>MGEEVNFDWHLLLNGYYYSPVDLEVEDIFEIVNQPMDGNCLYHSLACGMIEEQQPDSYKLIKEQVREAAGLFWDTTEETKTTGEDLNGYLARIMKPNEWGSSLEVNFFSQKAKVTVYIWHEDASKHCDYVVRYGEDPMLESINIMHRRNHYDYLKPRGNQRTAVVKSGSHHHHHH[4x]

One specific mechanism used by nairoviruses is the production of a deubiquitinating enzyme, termed the vOTU, that disrupts the innate immune response. Interestingly, the nairoviral L segment also encodes a viral homologue of the ovarian tumor protease (OTU) at the N-terminus. Instead, the vOTU’s primary function appears to be the reversal of post-translational modifications by ubiquitin (Ub) and the Ub-like protein interferon stimulated gene product 15 (ISG15). Each vOTU possesses a seven-stranded beta sheet as the core feature, with five major alpha helices framing the rest of the structure.

The vOTUs from DGKV, QYBV, and TAGV readily crystallized and were solved to 1.62 Å, 1.65 Å, and 2.05 Å, respectively. TAGV vOTU, on the other hand, prefers K63 and K11 to a greater extent, while not possessing as much activity towards K48. In TAGV vOTU, Trp73 fits between Leu86 and Thr79. Similarly, for TAGV vOTU Thr76 and Glu78 form electrostatic interactions with Gln110 and Tyr133, respectively. In TAGV vOTU, this pocket is largely hydrophobic possessing two tyrosines as well as a valine. Looking at X-ray crystal structures of the CCHFV and DUGV vOTUs bound to Ub reveals that Leu8 in particular has to be spatially accommodated in a pocket deep within the interaction interface. To confirm that this interaction with Leu8 is likewise involved in Ub binding with these other vOTUs, isothermal titration calorimetry (ITC) was performed using the TAGV vOTU to determine the relative binding efficiency of alanine and asparagine Ub mutants (Ub-L8A and Ub-L8N) compared to WT Ub. While WT Ub bound strongly with a dissociation constant (KD) of 11.5 ± 2.5 μM, Ub-L8A showed no detectable binding under similar conditions. As expected, the disruptive mutants I130R in QYBV and Y129R and V131R in TAGV completely knocked out the ability to process Ub-AMC, in keeping with a previous report demonstrating that the presence of arginine hindered ERVEV vOTU Ub activity. Making the reverse mutation in TAGV vOTU, H146R, essentially knocked out this activity suggesting this residue to have a key impact in diminishing FARV vOTU’s activity compared to other vOTUs.2-hydroxy-7-methoxy-5-methyl naphthoic acid | C13 H12 O4 | 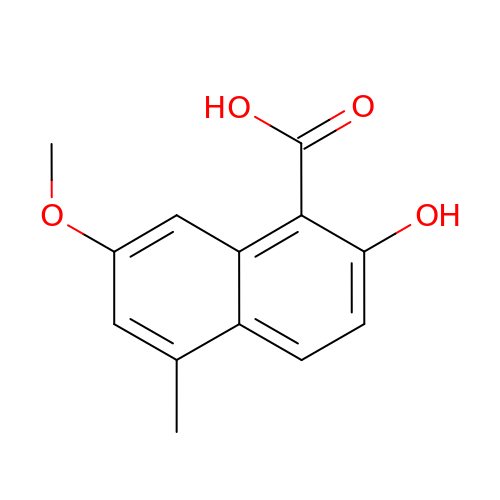LYGUXQMPYLCEGL-UHFFFAOYSA-N> MKHHHHHHHGAAGTSLYKKAGLVPRGSMNPQLYLCASVFITRGDVKSVSEIYQGLQSDAERLQYLKLLCVMWPELDAPTNISFVLKDIELNGMDESSVLVSLIQEDSSLTAISEMDVNTISKRVNALASYVEETLIGFNIHIRETHMLEDFIRARTLVVNSLSKDALCSLELLANSTSKSLVSWLDGILKPLDHLNRRLDTKLSIFQFENLSAQDAVSEMWKLPVKEVSVVRSMMKYEVEPYLKFQGSYTPFYEVIFNPDNFPLDSINNFQIYKYLSSQPTPLDTKFNETKWNILYSNGKNLASIPLPNLVFELESLIKS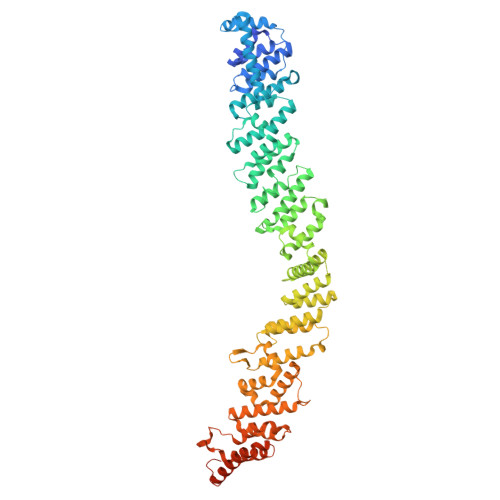FGDDSQIFSGISLNEWLVNLKFMNAMDIKDLKSLKKLQNEDSVVQTSYFSIITQNMFQGHIDIKTVQNVVEFIESSTLFDKLTNELQTSILLESLLKLGKFDILEQFVSTSGVKIQDKVIIQHFWRFFNIASNGSLSDPDMKNANRTLNLLSNKETHSNLYDILTIVDRLSHYSLSFKRGMPFKPAHISEFKANPMEIVEKLLDLNPKLRKNIEVTFDILKELYTALQVTPSDKDFTKEYSKLLSEHINNLLANGDFKFAFDQAINLIERPDAAEHWVTIFQVGKYIDPNWLDAEIPTEIIYLQLGIVSKLLHICPEKEYEVITSQWSGLELELSTRNLISDKYSLENTQRSNDNFMSDVSTNVGNFLSGKFQWNIGGA However, a freestanding enzyme D-aminoacyl-tRNA deacylase (DTD) removes D-amino acids (D-aas) mischarged on tRNAs and ensures that D-aas do not get incorporated into proteins. Mechanistically, the most remarkable challenge that DTD faces is to specifically act on multiple D-aa-tRNAs while rejecting L-aminoacyl-tRNAs (L-aa-tRNAs) without any specificity for either the amino acid or the tRNA. The enzyme is a symmetric dimer with two active sites per dimer that are located at the dimeric interface. A mechanistically unique solution to the problem of enantioselectivity employing two carbonyl oxygens from a ‘cross-subunit’ Gly-cisPro dipeptide has been shown to be responsible for D-chirality selection and strict L-chirality rejection from the active site of DTD.

PfDTD was co-crystallized with a post-transfer substrate analog D-Tyr3AA, which mimics D-tyrosine attached to the 3′-OH of the terminal adenosine (A76) of tRNA. The ester linkage between amino acid and adenosine is replaced by an amide linkage to make it non-hydrolyzable. Similar post-transfer substrate analogs have been used extensively to study proofreading mechanisms in atomic details for both Class I-specific CP1 editing domains and Class II-specific editing domains.The crystal structure of PfDTD in complex with D-Tyr3AA has been solved in two different crystal forms: crystal form I at a resolution of 1.86 Å in C2 space group and crystal form II at a resolution of 2.2 Å in P21 space group. Crystal forms I and II have two and eight copies per asymmetric unit, respectively. This provides us with 10 independent observations of the ligand in the active site. The superimposition of all the copies of ligand from both the crystal forms I and II shows considerable deviations in only the side chain atoms beyond Cβ. The lack of recognition of side chain atoms indicates that residues with different side chain chemistries and sizes are treated alike. Such a side chain-free recognition mechanism provides the basis for how nature has designed a single deacylase to deal with any D-aa-tRNA and reveals the crucial role played by weak hydrogen bonds in D-chirality selection. Therefore, the key to identifying the mechanism, as seen from this study, is the capturing of the D-Tyr3AA ligand that is bound in the actual substrate-binding pocket.

>[8x]MRVVIQRVKGAILSVRKENIGENEKELEIISEIKNGLICFLGIHKNDTWEDALYIIRKCLNLRLWNNDNKTWDKNVKDLNYELLIVSQFTLFGNTKKGNKPDFHLAKEPNEALIFYNKIIDEFKKQYNDDKIKIGKFGNYMNIDVTNDGPVTIYIDTHDINLNK N-[2-(oxidanylamino)-2-oxidanylidene-ethyl]-2-(4-sulfamoylphenyl)ethanamide 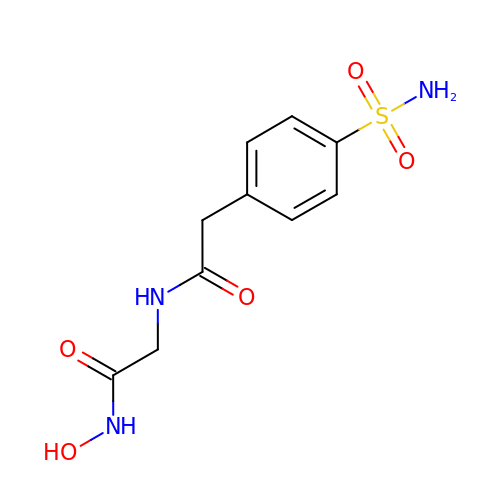| C10 H13 N3 O5 S | GWOXOVVAPORITL-UHFFFAOYSA-N>[4x]MKDIAIRGYCDRPSVATGETIRFYVSANETRGTFDAELVRLIHGDSNPAGPGYKEEAIKSDLEGQYPARFQRTQFGSYVEVADPDAGLQPDGAFSVHLFLWSTTPSRGRQGIASRWNDERQSGWNLAIEDGRVVFTIGDGSGATSSVVSDRPLFQQIWYSITGVYDPEKKQLRLYQKSVVNRTNSRFGLVVPLDSDCAVSADATVKAADSETSLLIAGLGEAAAQDGRTWCIAHYNGKVDAPKIYGCALGQDDAEKLSRGEIVRPISRLAHWDFSAGIGLNGIPTDHVVDASGYGHHGRCMNQPSRGSTGWNWDGHEENFIHCPEQYGALWFHEDCLDDCRWEKDFEFTVPEGLKSDFYAVKIRYEDTEDYIPFFVLPPRGTATAPILVIASTLSYLAYANEQIMHKADIGQAVAGHTPVLNENDVELHKNLSYYGLSTADGHIDGRGVQYTSWRRPIMNLRPKHRQGFGSIWELPADLHLIDWLNHNGFEYDVATEHDLNDQGAELLRRYKVVLTGSHPEYQTWANADAWEDYLADGGRGMYLAANGMYWIVEVHPEKPWVMEVRKELGVTAWEAPPGEYHYSTNGRRGGRFRGRARATQKIWGTGMSSFGFDHSGYFVQMPDSQDERVAWIMEGIDPEERIGDGGLVGGGAGGYELDRYDLALGTPPNTLLLASSVEHSVVYTVIPDDKAFPHPGMNGGEHPFVRADITYFSTANGGGMFATSSISWLGSLSWNDYDNNVSKMTKNVLNQFIKDEPAPRVKLAAALEHHHHHH;>[4x]MTEASESCVRDPSNYRDRSADWYAFYDERRRKEIIDIIDEHPEIVEEHAANPFGYRKHPSPYLQRVHNYFRMQPTFGRYYIYSEREWDAYRIATIREFGELPELGDERFKTEEEAMHAVFLRRIEDVRAELA

Certain bacterial species from genera such as Paracoccus, Pseudomonas, and Alcaligenes have evolved to use DMF as a sole carbon and nitrogen source for growth via degradation by a dimethylformamidase (DMFase). We show that DMFase from Paracoccus sp. strain DMF is a halophilic and thermostable enzyme comprising a multimeric complex of the α2β2 or (α2β2)2 type. The active site consists of a mononuclear iron coordinated by two Tyr side‐chain phenolates and one carboxylate from Glu. The Fe3+ ion in the active site catalyzes the hydrolytic cleavage of the amide bond in DMF.

The mutants Y440A and E521A were catalytically inactive. Structures of these mutant enzymes determined by cryoEM show a loss of Fe atoms. In the EM structures of the active site mutants (Y440A and E521A), the interface between the large and the small subunit becomes disordered, thus suggesting a role for the small subunit in the substrate entry pathway.> QRPEPTPEEWDLIHIATEAHRSTNAQGSHWKQRRKFLPDDIGQSPIVSMPDGDKVDLEAFSEFTKIITPAITR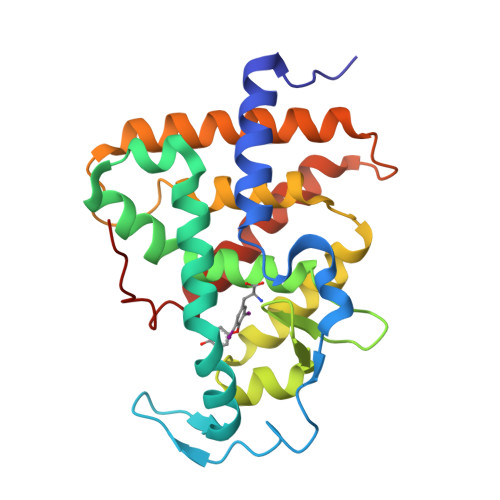VVDFAKKLPMFSELPCEDQIILLKGCCMEIMSLRAAVRYDPESDTLTLSGEMAVKREQLKNGGLGVVSDAIFELGKSLSAFNLDDTEVALLQAVLLMSTDRSGLLCVDKIEKSQEAYLLAFEHYVNHRKHNIPHFWPKLLMKVTDLRMIGACHASRFLHMKVE> MSFRYTNHLVATLKHRLFLEAAHRQLVRQTFTGVCNGIEVTCTAYGSVVGIRMLDRAVWEPHYQVAAD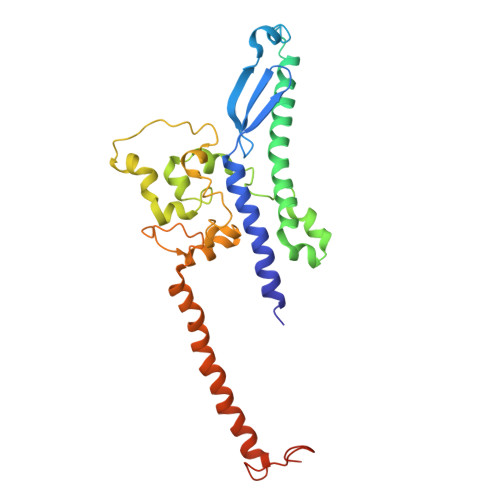NKSEAAAATPTAPAAASPSRPSSSSSSSSTASGKTGIDLVKLSASIQAATWQAIQKVRAAKEETHSRSLRRNPQVLAEARLRDWYEQDANTLHPRPFDGLKNLEATEWMQAVRFGVPQPARYRRPNAAPKDLGEGGDGAHTDQKPRETITVLRDEDCDPANIPIGSVHPLFAPGLLQLEVDPNVATNGGSRVDEFFVLSEQRKEMRRDEEAFWERVELIRRSQLATIPKGGVKRGYADMADTVQDSIEEKVQLRFTQ>MAIAHLATEYVFSDFLLKEPTEPKFKGLRLELAVDKMVTCIAVGLPLLLISLAFAQEISIGTQISCFSPSSFSARQAAFVDSYCWAAVQQKSSLQSESGNLPLWLHKFFPYILLLFAILLYLPALFWRFSAAPHLCSDLKFIMEELDKVYNRAIKAAKSARDLDLRDGPGPPGVTENVGQSLWEISESHFKYPIVEQYLKTKKNSSHLIMKYISCRLVTFVVILLACIYLSYYFSLSSLSDEFLCSIKSGVLKNDSTIPDRFQCKLIAVGIFQLLSLINLIVYALLIPVVVYTFFIPFRQKTDILKVYEILPTFDVLHFKSEGYNDLSLYN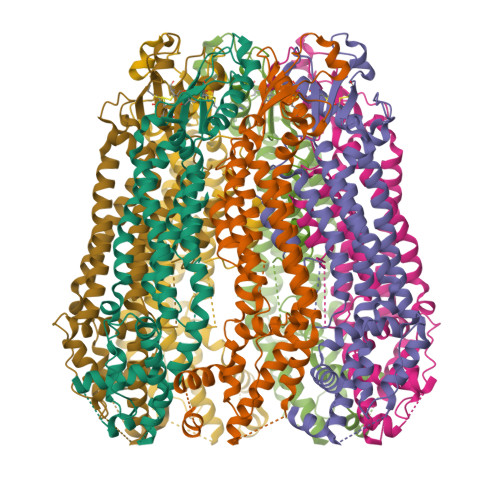LFLEENISELKSYKCLKVLENIKSNGQGIDPMLLLTNLGMIKMDIIDGKIPTSLQTKGEDQGSQRVEFKDLDLSSEAAANNGEKNSRQRLLNPSCGSAAAENLYFQGHHHHHH[7x]> SSLLSRLTQSNQSKDKIIAAL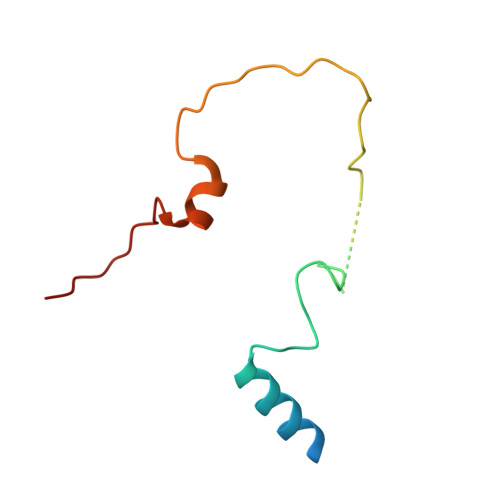AKRNVYKSFAGLYDSKGKNDNTGYDFDSNYARVGRHGSFILPVSKSVPTPSLLIEGSIVQRKNIKIE>TATDNARQVTIIGAGLAGTLVARLLARNGWQVNLFERRPDPRIETGARGRSINLALAERGAHALRLAGLEREVLAEAVMMRGRMVHVPGTPPNLQPYGRDDSEVIWSINRDRLNRILLDGAEAAGASIHFNLGLDSVDFARQRLTLSNVSGERLEKRFHLLIGADGCNSAVRQAMASVVDLGEHLETQPHGYKELQITPEASAQFNLEPNALHIWPHGDYMCIALPNLDRSFTVTLFLHHQSPAAQPASPSFAQLVDGHAARRFFQRQFPDLSPMLDSLEQDFEHHPTGKLATLRLTTWHVGGQAVLLGDAAHPMVPFHGQGMNCA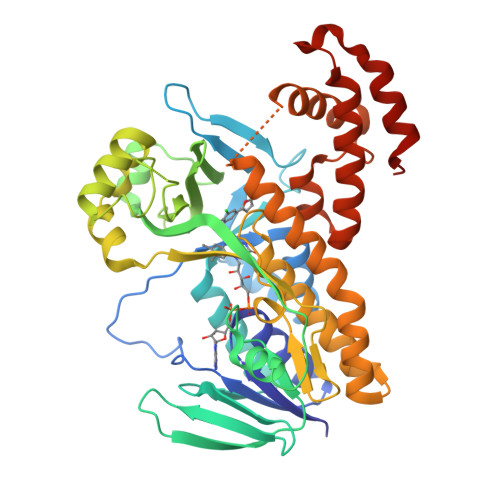LEDAVALAEHLQSAADNASALAAFTAQRQPDALAIQAMALENYVEMSSKVASPTYLLERELGQIMAQRQPTRFIPRYSMVTFSRLPYAQAMARGQIQEQLLKFAVANHSDLTSINLDAVEHEVTRCLPPLSHLS[2x]> 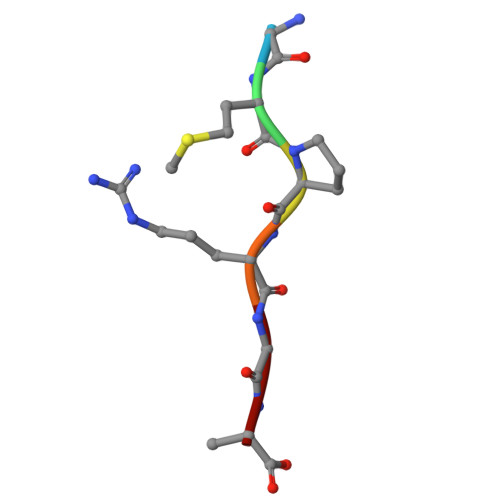GMPRGA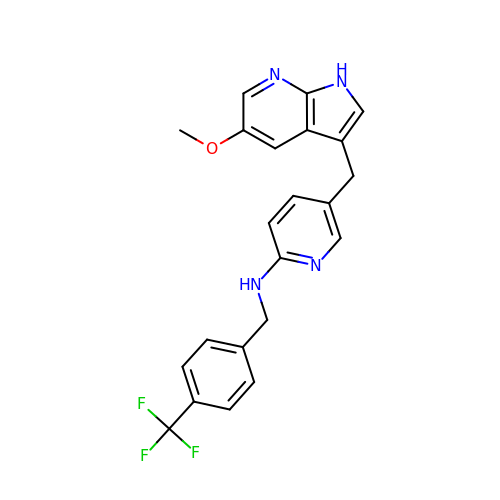5-[(5-methoxy-1H-pyrrolo[2,3-b]pyridin-3-yl)methyl]-N-[4-(trifluoromethyl)benzyl]pyridin-2-amine | C22 H19 F3 N4 O | WLYQGNIWNGFGPH-UHFFFAOYSA-N> MNPSPRKRVALFTDGACLGNPGPGGWAALLRFHAHEKLLSGGEACTTNNRMELKAAIEGLKALKEPCEVDLYTDSHYLKKAFTEGWLEGWRKRGWRTAEGKPVKNRDLWEALLLAMAPHRVRFHFVKG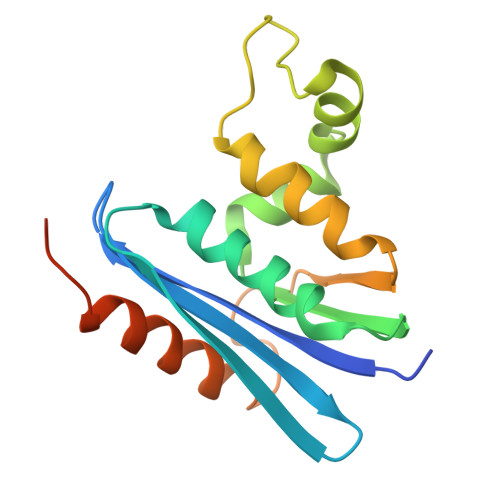HTGHPENERVDREARRQAQSQAKTPCPPRAPTLFHEEA N-[5-(6-methoxy-1H-indazol-5-yl)-1H-pyrazol-4-yl]pyrazolo[1,5-a]pyrimidine-3-carboxamide 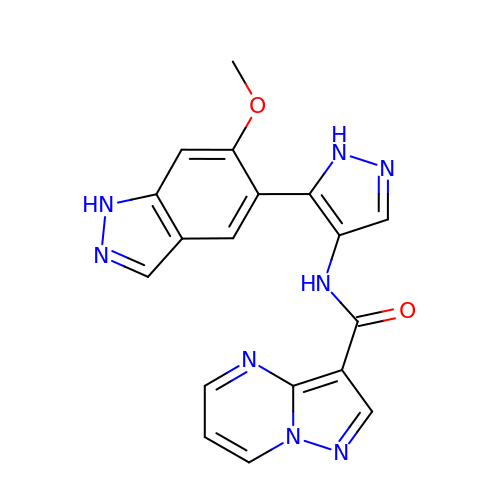| C18 H14 N8 O2 | YENOZGNVRCRNCQ-UHFFFAOYSA-N> MVWLNGEPRPLEGKTLKEVLEEMGVE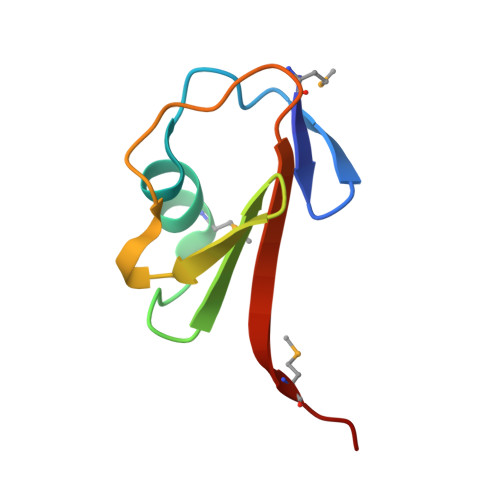LKGVAVLLNEEAFLGLEVPDRPLRDGDVVEVVALMQGG> MSSVEELTQLFSQVGFEDKKVKEIVKNKKVSDSLYKLIKETPSDYQWNKSTRALVHNLASFVKGTDLPKSELIVNGIINGDLKTSLQ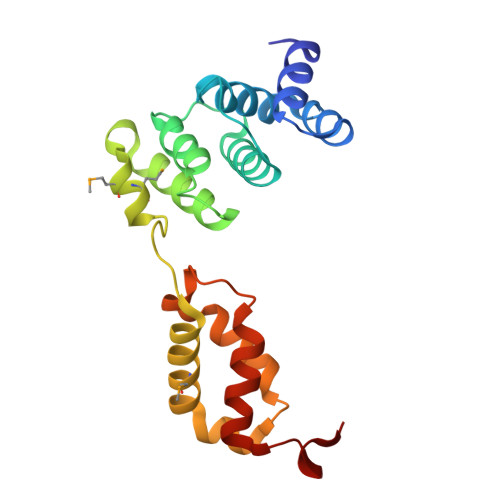VDAAFKYVKANGEASTKMGMNENSGVGIEITEDQVRNYVMQYIQENKERILTERYKLVPGIFADVKNLKELKWADPRSFKPIIDQEVLKLLGPKDERDLI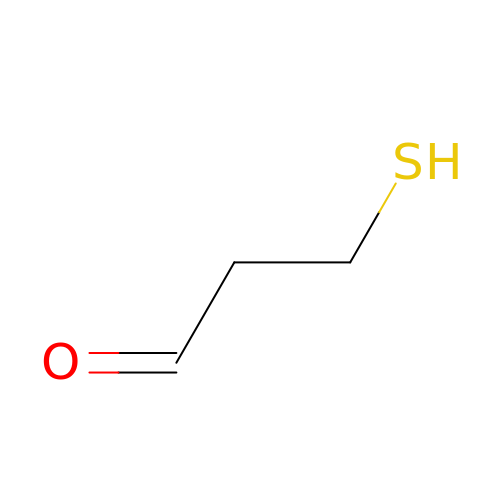2-MERCAPTO-PROPION ALDEHYDE | C3 H6 O S | BMYLOHDOJPEVOR-UHFFFAOYSA-N>[3x]SNAMNSQLTLRALERGDLRFIHNLNNNRNIMSYWFEEPYESFDELEELYNKHIHDNAERRFVVEDAQKNLIGLVELIEINYIHRSAEFQIIIAPEHQGKGFARTLINRALD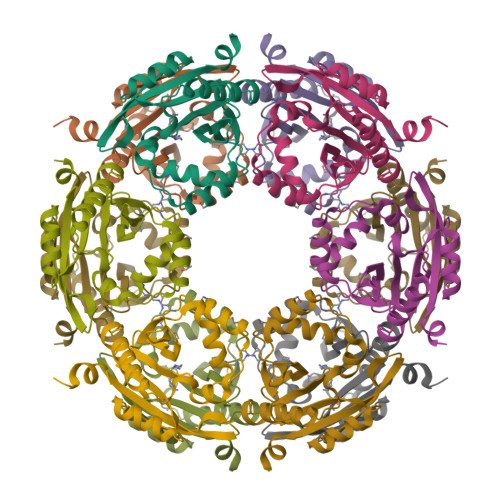YSFTILNLHKIYLHVAVENPKAVHLYEECGFVEEGHLVEEFFINGRYQDVKRMYILQSKYLNRSE> MGTVSSRRSWWPLPLLLLLLLLLGPAGARAQEDEDGDYEELVLALRSEEDGLAEAPEHGTTATFHRCAKDPWRLPGTYVVVLKEETHLSQSERTARRLQAQAARRGYLTKILHVFHGLLPGFLVKMSGDLLELALKLPHVDYIEEDSSVFAQSIPWNLERITPPRYSADEYQPPDGGSLVEVYLLDTSIQSDHREIEGRVMVTDFENVPEEDGTRFHRQASKCDSHGTHLAGVVSGRDAGVAKGASMRSLRVLNCQGKGTVSGTLIGLEFIRKSQLVQPVGPLVVLLPLAGGYSRVLNAACQRLARAGVVLVTAAGNFRDDACLYSPASAPEVITVGATNAQDQPVTLGTLGTNFGRCVDLFAPGEDIIGASSDCSTCFVSQSGTSQAAAHVAGIAAMMLSAEPELTLAELRQRLIHFSAKDVINEAWFPEDQRVLTPNLV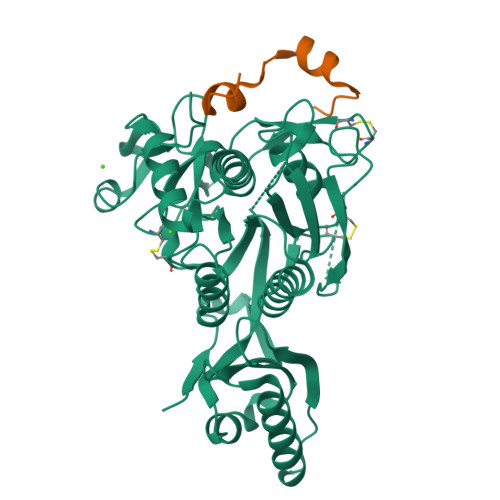AALPPSTHGAGNSHHHHHH;> TVFTSWEEYLDWVGSGDLMPWNLVRIGLLR(3S)-1-(1,3-BENZODIOXOL-5-YLMETHYL)-3-[4-(1H-IMIDAZOL-1-YL)PHENOXY]PIPERIDINE | C22 H23 N3 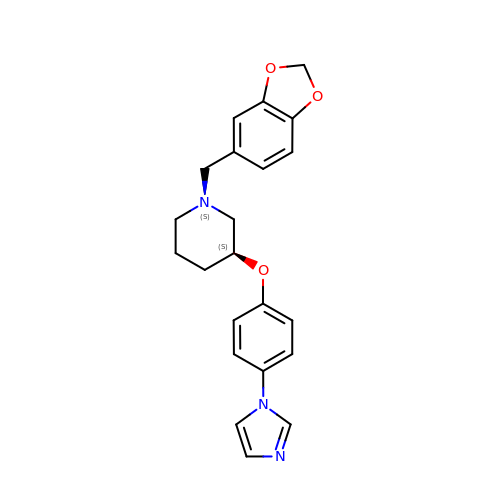O3 | HHOPJGKEAIIIDF-FQEVSTJZSA-N>[2x]MASNQELVQIATNFLLNAPPCEFMEVVSDVRALLPSESLLNASAGSTFREYNTSQMVSVQTSKGSALITKEGEISNNEYLDPKNKQVITYDHIKQEVTGERSASGEIEQDIEQYRAAFDEEATKYCNEYYPNGVSAVYGTKVSEGIKITVCISTCIYKPNAFYSGRWRSVWTCTFKPGSGNVTSNGKVQVNVHYFEDGNVQLNTVTQKQTTSPSADAQSTAVNAFKAIGKAELNLHTALDNNYSTMGDTTFKALRRALPINRTKINWQKVKNFKIANELNK;>MDHHHHHHHHTSETGYVQGTEKQLSCCLDLMRRLPPSQIEDNLAGLLDLVPDLTEDLLSSIDQPLKVAYDAVSKKDYLLCDYNRDADSYRSPWSNKYDPPLSGACYPSSKLRDIEVQANEIFEI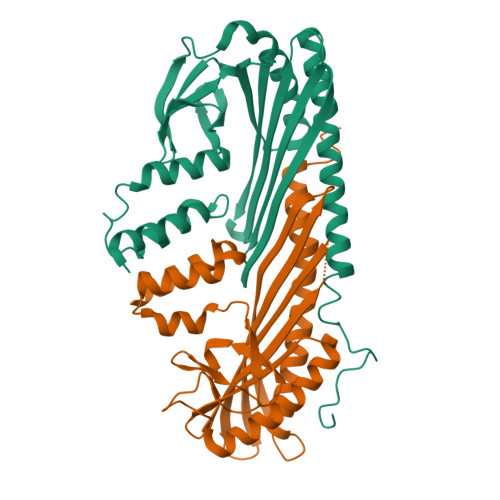YLNLYFEGGVSSVYCWDLDDNFAAVVLMKKTQDQSKKGQPMRGTWDSIHVVEVKLGKKDKAVYKLTSTVMLSIETDNDNTGKVNLAGSLTRQDEKEYTFNEVDTHCVNIGKMVEDMESKLRQTLETIYFGKTKEVVNTLRNATGNSELEKRKNLSNQIGSAIGNRG[2x]>GSQVDAEGNPFWEISDKRRVGISQFKKMDFINIREYYEAGGEMKPGKKGIGLTVDQYTAFLKAIPAINAELRSRGHDIT[6x]

Sub1 orthologous proteins, including the human PC4, have single-stranded DNA (ssDNA) binding, DNA unwinding activity and multiple functions in transcription and DNA repair. Nucleic acid binding is the key factor for Sub1's function in DNA-dependent processes such as transcription and DNA repair. F77 is conserved in all Sub1 orthologous proteins (Interpro domain IPR003173) of nine key species, while W89 is substituted by tyrosine in the proteins of six species (rice, mouse-ear cress, fruit fly, nematode, budding and fission yeast) as well as MoSub1 in Magnaporthe oryzae. In order to determine the effect of tryptophan/tyrosine substitutions of PC4 orthologous proteins, we have determined the crystal structures of the DNA complexes of the PC4 W89Y mutant and MoSub1 and analysed the effect of the W89Y mutation of PC4 on DNA binding affinity.

The structure of the MoSub1-DNA complex was determined at 2.7 Å resolution by molecular replacement. The asymmetric unit (ASU) comprises six protein molecules and three ssDNA chains. Each chain of ssDNA is bound by two monomers from two different dimers of MoSub1, which differs from the PC4-DNA complex in which PC4 binds to DNA with two monomers from the same dimer10. Nevertheless, the ssDNA is still bound by the same DNA-binding motif predicted by the apo- and PC4-DNA complex structures. Each protein subunit contains a curved five stranded anti-parallel β-sheet (β1-β5) followed by one α-helix, which is a key element in the dimer interface. When chain F of MoSub1 is superposed on the DNA-free structure, the RMSD of the Cα positions is ~1.0 Å, indicating that DNA binding induces little or no changes in the structure of MoSub1. The only distinct structural difference upon DNA binding is in the region of three loops (40, 60, and 70-loop), which are close to the DNA binding surface. The major interface with ssDNA (dT4 to 8) is formed by three β-strands (3–5) that are linked by the 60-loop and 70-loop and it appears that a number of residues in the interface, including F62, Y74, P82, S60, and N69, close in on the ssDNA upon interaction. Most of these interactions occur between the bases of ssDNA and aromatic residues, such as Y74 and F62 that are conserved in the PC4-DNA complex. Among them, Y74 of MoSub1 interacts with a single nucleotide in a similar way as Y89 of PC4 mutant.The biocatalytic reduction of the oxime moiety to the corresponding amine group has only recently been found to be a promiscuous activity of ene-reductases transforming α-oximo β-keto esters. By studying the crystal structures of enzyme oxime complexes, analyzing molecular dynamics simulations, and investigating biocatalytic cascades and possible intermediates, we obtained evidence that the reaction proceeds via an imine intermediate and not via the hydroxylamine intermediate. To gain more insight into the reaction pathway, we determined the crystal structures of the two enzymes OPR3 and XenA in complex with the oxime substrates 1a–c, either by co-crystallization or by soaking. All the crystal structures obtained had a high resolution (1.9–1.35 Å) and showed clear electron density features for the oximes.

To assess if the introduced amino acid exchanges affected the overall structure and the binding of the oxime, we also crystallized the tyrosine variants in complex with selected oxime substrates. The protomers in the crystal structures of the tyrosine variants are perfectly superimposable with the ones of the wild-type enzymes, confirming that the exchanges did not lead to major structural alterations. Interestingly, the binding mode of the oxime substrates also did not change in most of the structures. The propanoyl moiety of oxime 1b points into this cavity and is likely stabilized by hydrophobic interactions. Substrates with an acetyl moiety (such as oximes 1a and 1c) give the non-productive binding mode described above. Testing the tyrosine variants for oxime reduction showed that the exchange of the non-canonical tyrosine Y370 to phenylalanine in OPR3 led to significantly decreased product formation compared to the wild type (OPR3_Y370F). In comparison to the wild type, the non-canonical tyrosine variant Y370F of OPR3 showed a 4-fold decrease in both kred and Kd in the reductive half-reaction and a 3- and 2-fold decrease in kox and Kd in the oxidative half-reaction. The effect of the Y370F mutation on the oxidative half-reaction is a clear indication that this residue has a role in the catalytic mechanism. The non-canonical tyrosine residue Y370 was shown to contribute to the reduction of the oxime moiety most likely via protonation of the hydroxy/methoxy moiety, leading to the imine intermediate.

>MASSAQDGNNPLFSPYKMGKFNLSHRVVLAPMTRCRALNNIPQAALGEYYEQRATAGGFLITEGTMISPTSAGFPHVPGIFTKEQVREWKKIVDVVHAKGAVIFCQLWHVGRASHEVYQPAGAAPISSTEKPISNRWRILMPDGTHGIYPKPRAIGTYEISQVVEDYRRSALNAIEAGFDGIEIHGAHGYLIDQFLKDGINDRTDEYGGSLANRCKFITQVVQAVVSAIGADRVGVRVSPAIDHLDAMDSNPLSLGLAVVERLNKIQLHSGSKLAYLHVTQPRYVAYGQTEAGRLGSEEEEARLMRTLRNAYQGTFICSGGYTRELGIEAVAQGDADLVSYGRLFISNPDLVMRIKLNAPLNKYNRKTFFTQDPVVGYTDYPFLQGNGSNGPLSRLLEHHHHHH[2x]>NAMVVTLDGEILQPGMPLLHADDLAAVRGDGVFETLLVRDGRACLVEAHLQRLTQSARLMDLPEPDLPRWRRAVEVATQRWVASTADEGALRLIYSRGREGGSAPTAYVMVSPVPARVIGARRDGVSAITLDRGLPADGGDAMPWLIASAKTLSYAVNMAVLRHAARQGAGDVIFVSTDGYVLEGPRSTVVIATDGDQGGGNPCLLTPPPWY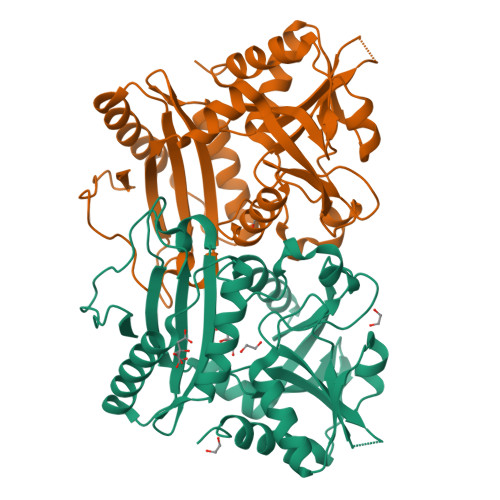PILRGTTQQALFEVARAKGYDCDYRALRVADLFDSQGIWLVSSMTLAARVHTLDGRRLPRTPIAEVFAELVDAAIVSDR[2x]> 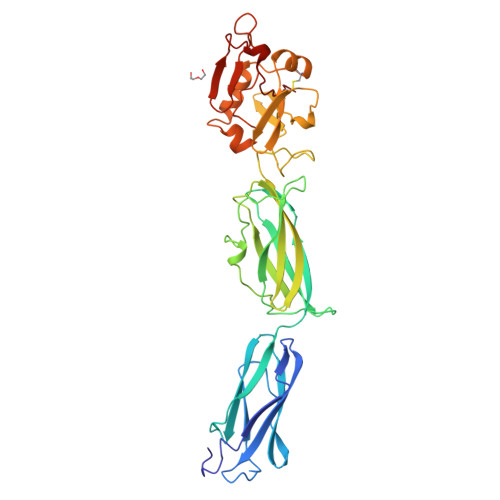GGGRGNLSTTNSTLVAAPVNIEANGSDTSVVTLTLRDSNNNPVTGQTVAFTSTLGTLDNVTEQASGLYTATLTAGTLTGTASLSVNVDGNNLGTTPATINVIPAPVDLTVLTDNARKNIGQAISLTVIAKYKSTDVVAPNVKMTFEQVAVVNRQNSPVSSSGVVQIADANYDAFTGMTDANGQLTVSVTDPNGIGVQTTLRAAAESGDMENTNVTFNVITSPDSAQASMWGNMAETLTASGVTFKRPYLAAEKPGTIGTNVENNETWAMFNQSQAVAMCTVPSSSQLVSLYNLYPLNQIQTVAGWPTMQVYRSSTSAVIGQHFYVYMNTGNYAYNSIGNGDVDGNYNVSCSL> MSKESSVAPTERVNIVYKPATGNAQEQVELPLKVLMLGDFTGQEDARPLEQRAPINVDKANFNEVMAQQNLKVTLTAADKLSADPNATMNVSLQFKNLNDFSPESVVN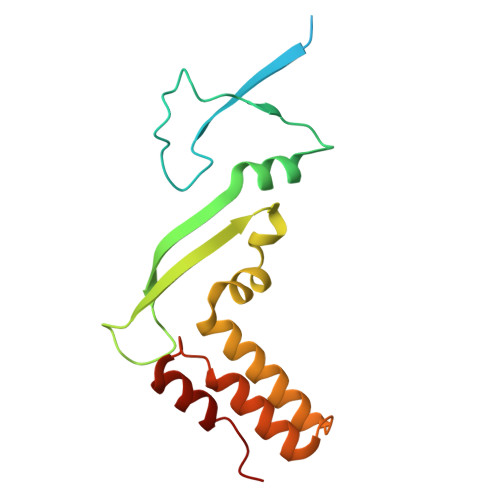QVPELKKLLELRSALNALKGPLGNLPAFRKKLQALLADEDGRKALIKELGLTEETK> MLKDLLNLLKNQGQIEEFDAIRIGLASPEMIRSWSFGEVKKPETINYRTFKPERDGLFCAKIFGPVKDYECLCGKYKRLKHRGVICEKCGVEVALAKVRRERMGHIELASPVAHIWFLKSLPSRIGLLLDMTLRDIERVLYFESYVVIDPGMTTLEKGQLLNDEQYFEALEEFGDDFDARMGAEAVHELLNAIDLEHEIGRLREEIPQTNSETKIKKLSKRLKLMEAFQGSGNKPEWMVLTVLPVLPPDLRPLVPLDGGRFATSDLNDLYRRVINRNNRLKRLLDLAAPDIIVRNEKRMLQEAVDALLDNGRRGRAITGSNKRPLKSLADMIKGKQGRFRQNLLGKRVDYSGRSVITVGPTLRLHQCGLPKKMALELFKPFIFGKLEGRGMATTIKAAKKMVERELPEVWDVLAEVIREHPVLLNRAPTLHRLGIQAFEPVLIEGKAIQLHPLVCAAYNADFDGDQMAVHVPLTLEAQLEARALMMSTNNILSPANGEPIIVPSQDVVMGLYYMTREAINAKGEGMAFADLQEVDRAYRSGQASLHARVKVRINEKIKGEDGQLTANTRIVDTTVGRALLFQVVPAGLPFDVVNQSMKKKAISKLINHCYRVVGLKDTVIFADQLMYTGFAYSTISGVSIGVNDFV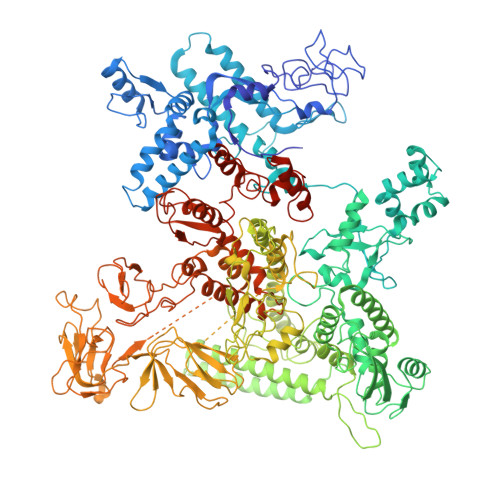IPDEKARIINAATDEVKEIESQYASGLVTQGEKYNKVIDLWSKANDEVSKAMMANLSKEKVVDREGKEVDQESFNSMYMMADSGARGSAAQIRQLAGMRGLMAKPDGSIIETPITANFREGLNVLQYFISTHGARKGLADTALKTANSGYLTRRLVDVAQDLVVTEIDCGTEHGLLMSPHIEGGDVVEPLGERVLGRVIARDVFKPGSDEVIVPAGTLIDEKWVDFLEVMSVDEVVVRSPITCETRHGICAMCYGRDLARGHRVNIGEAVGVIAAQSIGEPGTQLTMRTFHIGGAASRTSAADNVQVKNGGTIRLHNLKHVVRADGALVAVSRSGELAVADDFGRERERYKLPYGAVISVKEGDKVDPGAIVAKWDPHTHPIVTEVDGTVAFVGMEEGITVKRQTDELTGLTNIEVMDPKDRPAAGKDIRPAVKLIDAAGKDLLLPGTDVPAQYFLPANALVNLTDGAKVSIGDVVARIPQETSKTRDITGGLPRVADLFEARRPKEPSILAEISGTISFGKETKGKRRLVITPNDGSDPYEELIPKWRHLNVFEGEQVNRGEVISDGPSNPHDILRLLGVSSLAKYIVNEIQDVYRLQGVKINDKHIETILRQMLRKVEVSESGDSSFIKGDQVELTQVLEENEQLGTEDKFPAKYERVLLGITKASLSTESFISAASFQETTRVLTEAAVTGKRDFLRGLKENVVVGRLIPAGTGLAYHSERKRQRDLGKPQRVSASEAEAALTEALNSSGNGSGSWSHPQFEK> MGHHHHHHMRSYEKSKTAFKEAQKLMPGGVNSPVRAFKSVDMDPIFMERGKGSKIFDIDGNEYIDYVLSWGPLILGHTNDRVVESLKKVAEYGTSFGAPTEVENELAKLVIDRVPSVEIVRMVSSGT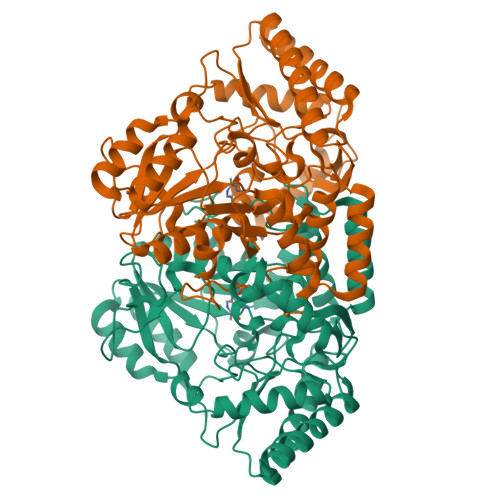EATMSALRLARGYTGRNKILKFEGCYHGHGDSLLIKAGSGVATLGLPDSPGVPEGIAKNTITVPYNDLESVKLAFQQFGEDIAGVIVEPVAGNMGVVPPQEGFLQGLRDITEQYGSLLIFDEVMTGFRVDYNCAQGYFGVTPDLTCLGKVIGGGLPVGAYGGKAEIMEQIAPSGPIYQAGTLSGNPLAMTAGLETLKQLTPDSYKNFIKKGDRLEEGISKAAEAHGIPHTFNRAGSMIGFFFTNEPVINYETAKASDLKLFASYYKGMANEGVFLPPSQFEGLFLSTAHTDEDIENTIQAAEKVFAEISRR>MKRVVVTGMAGITSLGETADDIFARFEAGKSGIRYMPEWEQYVDLRTKLAGPVETFHIPKHFNRKVTRGMGRVALMSVVCAETALQNAGLLGHEILSSGEAGVAFGSSAGSVDAVGEFASMLLHQSMSKINATTYIRMMAHTSAVNMTVYFGLKGLTLPTSSACTSGSMAIGQAYEAIKYGKQQVMIAGGAEELSAAGAAVFDVLFATSGMNDQPEKTPRPFDAKRDGLVIGEGAGCLILEEYEHAKARGAHIYAEVIGYGSNTDGQHVTRPESEMMGRCMELALKDASVEAKDIAYVNAHGTSTDQGDVAESQATAKVLGYKPISSLKSYFGHTLGACGAIEAWLSIEMMNRGRFIPTLNLDEIDSLCGELDYIVQQPRNLDADIIMSNNFAFGGINTSLIFKRVKQ[4x]

Aryl polyenes (APE) are one of the most widespread secondary metabolites among gram-negative bacteria. APE biosynthesis gene clusters harbor two ketosynthases (KSs): the heterodimeric KS-chain length factor complex, ApeO-ApeC, and the homodimeric ketoacyl-acyl carrier protein synthase I (FabB)-like KS, ApeR. To understand the structural basis of the functional redundancy in the two KSs, AbApeO-AbApeC and AbApeR, from the APE BGC of A. baumannii, we determined the crystal structures of AbApeO-AbApeC and AbApeR in the absence of substrates. Therefore, the two KSs function complementarily in the generation of APE to enhance its production.

The crystal structure contained four molecules of AbApeR in the asymmetric unit. AbApeR was a homodimeric protein with twofold symmetry, and there were two homodimers in the crystal structure. AbApeR and E. coli KAS I protein (EcFabB) were remarkably similar. The proteins shared an amino acid sequence identity of 39% and the proteins could be superposed with an r. m. s. d. of 0.886 Å. The cavity of AbApeR was symmetrical and connected between the homodimeric partners, forming an elongated, narrow canal across the dimer. The residues lining the cavity of AbApeR were moderately hydrophobic. The volume of the cavity was 120 Å3, which was considerably similar to that of the AbApeO-AbApeC heterodimer. The cavity volume of AbApeR near the entrance is reduced, when compared to that of AbApeO-AbApeC, because of the presence of Tyr135. Mutagenesis at Tyr135 in the active site cavity of ApeR reduces the activity significantly, which suggests that the stacking of the aryl group between Tyr135 and Phe202 is important for substrate recognition. In the model of 3EN-AbApeR, the narrow binding site of 3EN moiety led to a dead end with approximately the length of three-double-bond polyene.6-{[(3R,4R)-4-(3-phenoxyphenoxy)pyrrolidin-3-yl]methyl}pyridin-2-amine | C22 H23 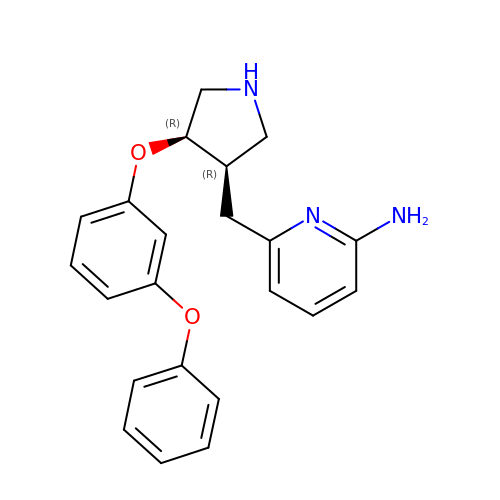N3 O2 | MKBQBMWQPUXDQQ-IERDGZPVSA-N> MSNISRQAYADMFGPTVGDKVRLADTELWIEVEDDLTTYGEEVKFGGGKVIRDGMGQGQMLAADCVDLVLTNALIVDHWGIVKADIGVKDGRIFAIGKAGNPDIQPNVTIPIGAATEVIAAEGKIVTAGGIDTAIHWICPQQAEEALVSGVTTMVGGGTGPAAGTHATTCTPGPWYISRMLQAADSLPVNIGLLGKGNVSQPDALREQVAAGVIGLKIHEDWGATPAAIDCALTVADEMDIQVALHSDTLNESGFVEDTLAAIGGRTIHTFHTEGAGGGHAPDIITACAHPNILPSSTNPTLPYTLNTIDEHLDMLMVCHHLDPDIAE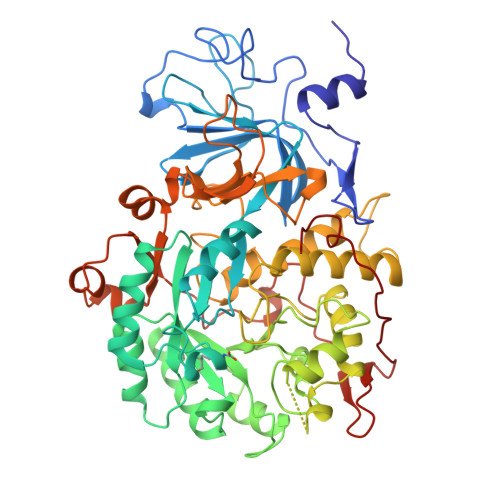DVAFAESRIRRETIAAEDVLHDLGAFSLTSSDSQAMGRVGEVILRTWQVAHRMKVQRGALAEETGDNDNFRVKRYIAKYTINPALTHGIAHEVGSIEVGKLADLVVWSPAFFGVKPATVIKGGMIAIAPMGDINASIPTPQPVHYRPMFGALGSARHHCRLTFLSQAAAANGVAERLNLRSAIAVVKGCRTVQKADMVHNSLQPNITVDAQTYEVRVDGELITSEPADVLPMAQRYFLF Cyclodipeptide synthases (CDPSs) use aminoacylated tRNA (aa-tRNA) substrates to form peptide bonds between two amino acids yielding a cyclic dipeptide product (CDP). ParaCDPS from Parabacteroides sp. 20_3 (GenBank: EFK64745.1) produces cyclo(His-Phe)8 whilst ParcuCDPS from Parcubacteria bacterium RAAC4_OD1_1 (GenBank: ETB63777.1) can synthesise both cyclo(His-Glu) and cyclo(His-Pro)9. ParcuCDPS belongs to the XYP sub-group of the CDPS family, characterised by the presence of 3 residues: X40 where X is a non-conserved residue, Y202, and P203 (numbering respective to AlbC). ParcuCDPS displays a Rossman-fold common throughout the CDPS family.

Inspired by HisRS and histidine recognition more generally, and by the only high resolution structure of a CDPS with a ligand bound, we systematically altered three unique residues in ParcuCDPS P1, which we hypothesised to be participating in crucial interactions with the polar side chain of histidine. We first designed Generation 1 containing seven P1 mutants (Y55F; Y55V; E174A; E174H; E174L; Y189F and Y189L), and these variants were cloned, expressed in E.coli, purified and used for activity assays. From these calculations, P1 is predicted to be mostly neutral apart from Tyr55 and Glu174 which form a negatively charged microenvironment, while P2 is predicted to be mostly lined by positively charged residues. By mutating the P1 residues, the activity of the variants was vastly reduced with E174A and E174H incapable of tolerating histidine as a substrate. E174A removed the hydrogen bonding network thought to be essential for steering histidine into the pocket whilst E174H was designed to reverse the charge of the residue and was predicted to repel the incoming histidine from P1. Further investigation into the changes imposed by these mutants was performed by solving the crystal structures of a select few mutants containing changes to the active site or the pocket residues. The mutant structures were able to be solved using WT as a model and retained an equivalent fold to ParcuCDPS (Supplementary Notes 4 and 7 relating to Supplementary Figs. 13 and 14). Therefore, the disruption of activity is caused exclusively by the change in these few residues which appear important for the enzyme to produce a CDP.

> MELHQIRGCHKNDIELKKYNIGVAISLGNKWFSIDNIEKLVKWSLLHTKEYVIIYIADSIHGINLSVRNKLSDSHAEEVAIRYGRNLFIKIKERVSLSFSQDEQAKIIYATWSDIADSKYKEKVKYLYNLYDKNINFKNYIENFVKEWVSKEKRTFNNNEINKFGRYILEELPALMVQVKARGVLFEAYVYPYKTRITEFVGLLQKGEIFPEIKTNILDNHPKIFLEVRE> MTSRKKVLLKVIILGDSGVGKTSLMNQYVNKKFSNQYKATIGADFLTKEVMVDDRLVTMQIWDTAGLERFQSLGVAFYRGADCCVLVFDVTAPNTFKTLDSWRDEFLIQASPRDPENFPFVVLGNKIDLENRQVATKRAQAWCYSKNNIPY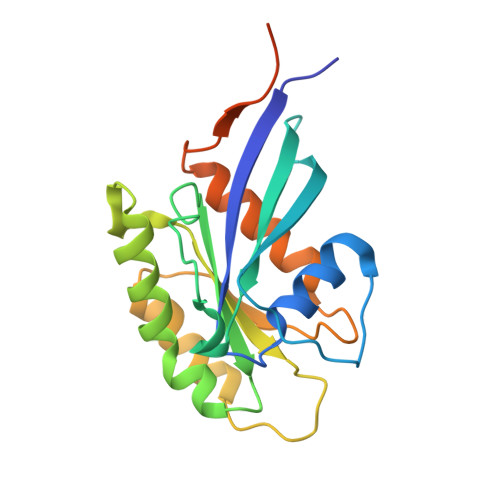FETSAKEAINVEQAFQTIARNALKQETEVELYNEFPEPIKLDKNDRAKASAESCSC>SNAIAAGGSHVEAAPQEEWKKHFIHTGELGSAEFASVMSHTTSAMKSVFEQVNAPYSGMDPKALEDAINAVDLDNKNAPLKSVIDDVAELVAKNAIFTQHPDCIAHLHTPPLMPAVAAEAMIAALNQSMDSWDQASSATYVEQKVVNWLCDKYDLSEKADGIFTSGGTQSNQMGLMLARDWIADKLSGHSIQKLGLPDYADKLRIVCSKKSHFTVQKSASWMGLGEKAVMTVDANADGTMDITKLDEVIAQAKAEGLIPFAIVGTAGTTDHGAIDDLDFIADMAVKHDMWMHVDGAYGGALILSSHKSRLKGVERAHSISVDFHKLFYQTISCGALLVNDKSNFKFLLHHADYLNREHDELPNLVDKSIATTKRFDALKVFMTMQNVGPKALGDMYDHLLAQTLEVADMIRTNDQFELLAEPSLSTVLFRATHETADLDELNKALRLEALTRGIAVLGETIVDGKTALKFTILNPCLTTSDF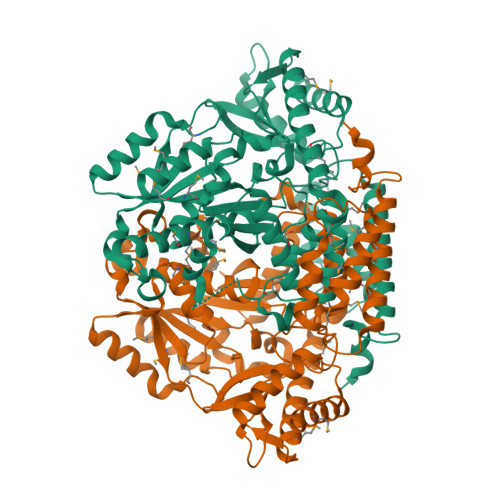ESLLSKINMLAVELV[2x]(R)-4-[2-(3-AMINO-BENZENESULFONYLAMINO)-1-(3,5-DIETHOXY-2-FLUOROPHENYL)-2-OXO-ETHYLAMINO]-2-HYDROXY-BENZAMIDINE | C25 H28 F N5 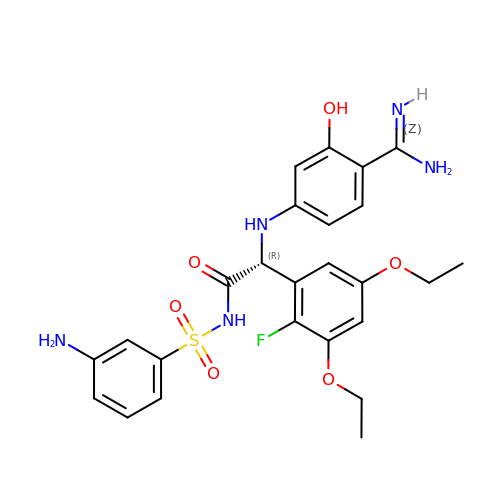O6 S | MLPXCKVDBGAVRJ-HSZRJFAPSA-N The re-acylation is catalyzed by lysophosphatidylcholine acyltransferase (LPCAT) and among the four LPCAT members in human, the LPCAT3 preferentially introduces polyunsaturated acyl onto the sn-2 position of lysophosphatidylcholine, thereby modulating the membrane fluidity and membrane protein functions therein. Combining the x-ray crystallography and the cryo-electron microscopy, we determined the structures of LPCAT3 in apo-, acyl donor-bound, and acyl receptor-bound states. A reaction chamber was revealed in the LPCAT3 structure where the lysophosphatidylcholine and arachidonoyl-CoA were positioned in two tunnels connected near to the catalytic center. The structural and functional analysis provides the basis for the re-acylation of lysophosphatidylcholine and the substrate preference during the reactions.

Similar data collections and refinement processes were conducted on the cLPCAT3 samples supplemented with 0.5 mM 1-dodecanoyl-sn-glycero-3-phosphocholine (12:0-LPC) and EM maps were generated at an overall resolution of 3.57 Å. In the cryo-EM map for cLPCAT3/LPC was identified a large non-protein electron density located in the horizontal tunnel with no overlap with the araCoA electron density found in the EM map for cLPCAT3/araCoA. The C12:0-LPC molecule fits well in the density with the phosphorylcholine head positioned in the C-wing side and stabilized by the interactions with a series of hydroxy groups from tyrosine Y143, Y151, Y298, and Y394. When the interactions were impaired by the mutations of those tyrosine residues, the enzymatic activities of cLPCAT3 reduced significantly. The C12:0-acyl at sn-1 of the LPC extends to the N-wing side of the horizontal tunnel and ends near to the lateral gate formed by TM1 and 6, where the binding of acyl chain is mediated by its hydrophobic interaction with residues L58, I59, Y151, I153, L155, and V213. The sn-2 hydroxy of the glycerol backbone sits in close proximity to the catalytic residue H388, ready to be activated into a nucleophilic reagent through the deprotonation by the imidazolyl of the histidine. Interestingly, despite the empty vertical tunnel in our EM map for acyl receptor-bound state (cLPCAT3/LPC), a long, lipid-like density was revealed in the side pocket which meets the electron density of LPC at the joint point near to H388. Manually modeling the acyl of LPC into the density failed to generate well-fit models, suggesting this lipid-like density might not represent an alternative conformation of LPC molecules bound. Based on the absence of density corresponding to the CoA moiety, we speculated that this unmodeled density, in combination with the large density for LPC, might represent the PC product partially bound and co-purified with the protein.

>[2x]MGAERDESGAGAAVLVPLLGFGSNRPAGPAEKMAVAGSGWSLARVAEALGSSEQALRLIVSILMGYPFALFQRYFLFQKETYLIHLYNVFTGLSIAYFNFGMQFFHSLLCVLIQFLILRLMGRTVTAVFTTFVFQMTYLMAGYYFTATEHYDIKWTMPHCVLTLKLIGLAIDYYDGGKDPELLTPEQRRFAVRGVPTLLEVSGFSYFYGAFMVGPQFSMTDYQKLAKGEMTDVPGQRPNSFVPALKRLSLGLLFLVTYTLSSPYISEEYLISDDYMEKPFWFRCGYILVWGKIILYKYVTCWLVTEGVCILVGLGYNGNDQNGKPVWDACANMKVWLYETTPLFTGTIASFNINTNAWVARYVFKRLKFLGNKLLSQALALFFLAIWHGLHSGYLVCFQMELLIVIVERQVINLVRDSPTLSTLASITALQPIFYVLQQTNHWMFMGYSLVPFCLFTWDKWMKVYKSIYFLGHVLFFTLLLVLPYIRKLLVPRKEKLKKAE> MSTLQRRRVNRADSGDTSSIHSSANNTKGDKIANIAVDGDDDNGTNKKIAYDPEESKLRDNINIPTLTLMEEVLLMGLRDREGYLSFWNDSISYALRGCIIIELALRGKIRILDDSARKRFDLSERLIEVIDSSKTGEVLLDETLQLMKNDEPLSISNWIDLLSGETWNLLKINYQLKQVRERLAKGLV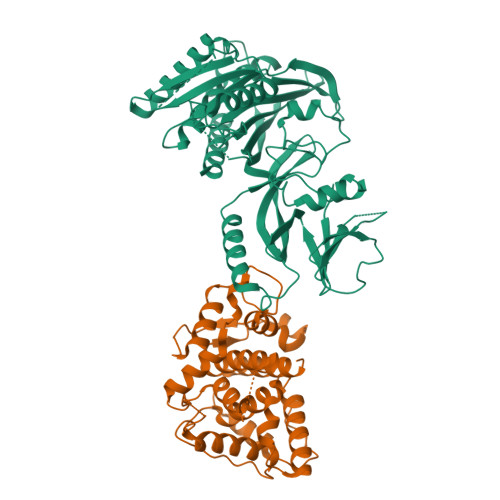DKGVLRTEMKNFFLFDMATHPIADASCKEAIKRRVLSVLVSRNMELSYNEYFPETTSFKIIRTLALICGSYGANVLENVLTTLEYEKRDKAISRAEEIMAQFSQYPFDLEKETELGVSVNLNKEVKEEIENNPGHDLQLEVIAGVFEVFSRMDMLL;> MTGPIVYVQNADGIFFKLAEGKGTNDAVIHLANQDQGVRVLGAEEFPVQGEVVKIASLMGFIKLKLNRYAIIANTVEETGRFNGHVFYRVLQHSIVSTKFNSRIDSEEAEYIKLLELHLKNSTFYFSYTYDLTNSLQRNEKVGPAASWKTADERFFWNHYLTEDLRNFAHQDPRIDSFIQPVIYGYAKTVDAVLNATPIVLGLITRRSIFRAGTRYFRRGVDKDGNVGNFNETEQILLAENPESEKIHVFSFLQTRGSVPIYWAEINNLKYKPNLVLGENSLDATKKHFDQQKELYGDNYLVNLVNQKGHELPVKEGYESVVHALNDPKIHYVYFDFHHECRKMQWHRVKLLIDHLEKLGLSNEDFFHKVIDSNGNTVEIVNEQHSVVRTNCMDCLDRTNVVQSVLAQWVLQKEFESADVVATGSTWEDNAPLLTSYQNLWADNADAVSVAYSGTGALKTDFTRTGKRTRLGAFNDFLNSASRYYQNNWTDGPRQDSYDLFLGGFRPHTASIKSPFPDRRPVYIQLIPMIICAALTVLGATIFFPKDRFTSSKNLLYFAGASIVLALSTKFMFKNGIQFVNWPKLVDVGFLVVHQTHDKEQQFKGLKYAQSPKFSKPDPLKRD>MSISISYSTTYSGWTVADYLADWSAYFGDVNARPGQVVDGSNTGGFNPGPFDGSQYALKSTASDAAFIAGGDLHYTLFSNPSHTLWGKLDSIALGDTLTGGASSGGYALDSQEVSFSNLGLDSPIAQGRDGTVHKVVYGLMSGDSSALQGQIDALLKAVDPSLSINSTFDQLAAAGVA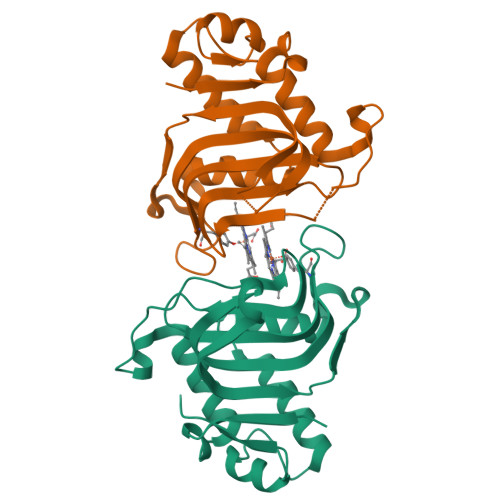HATPAA[2x]>RAPAPATPHAPDHSPAPNSPTLTRPPEGPKFPRVKNWELGSITYDTLCAQSQQDGPCTPRRCLGSLVLPRKLQTRPSPGPPPAEQLLSQARDFINQYYSSIKRSGSQAHEERLQEVEAEVASTGTYHLRESELVFGAKQAWRNAPRCVGRIQWGKLQVFDARDCSSAQEMFTYICNHIKYATNRGNLRSAITVFPQRAPGRGDFRIWNSQLVRYAGYRQQDGSVRGDPANVEITELCIQHGWTPGNGRFDVLPLLLQAPDEAPELFVLPPELVLEVPLEHPTLEWFAALGLRWYALPAVSNMLLEIGGLEFSA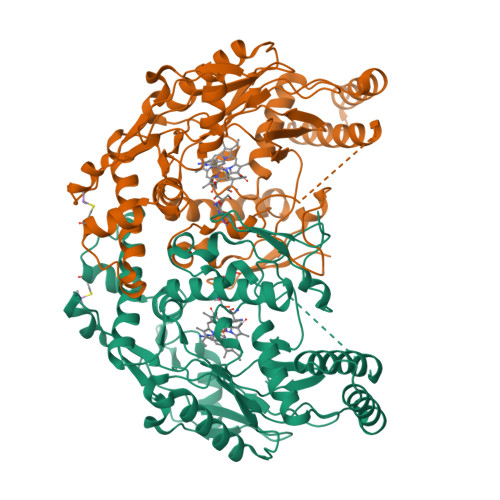APFSGWYMSTEIGTRNLCDPHRYNILEDVAVCMDLDTRTTSSLWKDKAAVEINLAVLHSFQLAKVTIVDHHAATVSFMKHLDNEQKARGGCPADWAWIVPPISGSLTPVFHQEMVNYILSPAFRYQPDPW[2x]1,5-dimethyl-3-oxidanyl-~{N}-[2,3,5,6-tetrakis(fluoranyl)-4-phenyl-phenyl]pyrazole-4-carboxamide 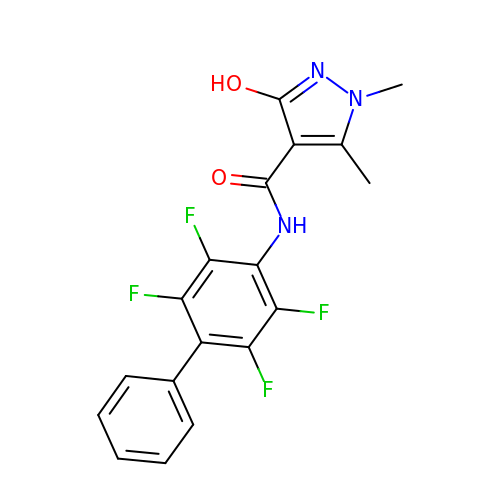| C18 H13 F4 N3 O2 | YELPXAASZKFOBT-UHFFFAOYSA-N>[2x]GHMSPNYDKWEMERTDITMKHKLGGGQYGEVYEGVWKKYSLTVAVKTLKEDTMEVEEFLKEAAVMKEIKHPNLVQLLGVCTREPPFYIITEFMTYGNLLDYLRECNRQEVN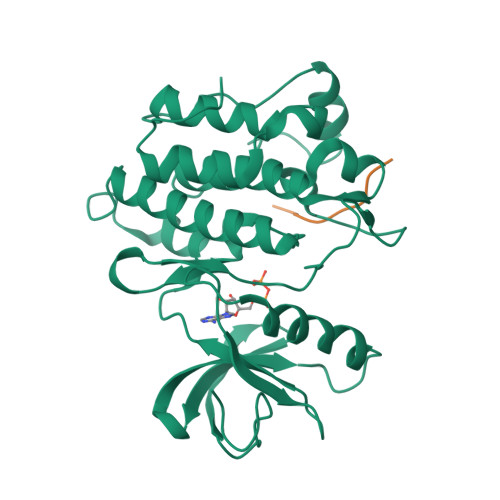AVVLLYMATQISSAMEYLEKKNFIHRDLAARNCLVGENHLVKVADFGLSRLMTGDTYTAPAGAKFPIKWTAPESLAYNKFSIKSDVWAFGVLLWEIATYGMSPYPGIDLSQVYELLEKDYRMERPEGCPEKVYELMRACWQWNPSDRPSFAEIHQAFETMFQESSISDEVEKELGK;>[2x]AEEEIFGEFEAKK> GHMDQETIDTDYDVIVLGTGITECILSGLLSVDGKKV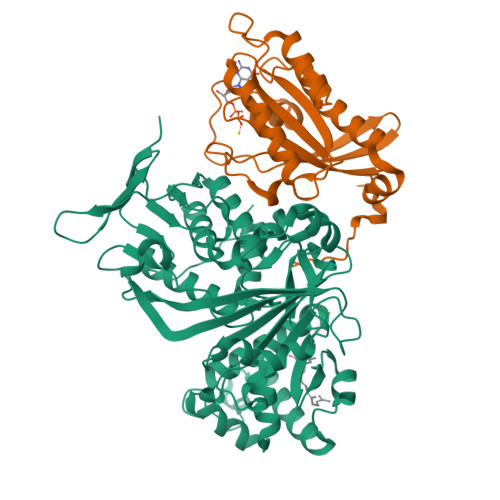LHIDKQDHYGGEAASVTLSQLYEKFKQNPISKEERESKFGKDRDWNVDLIPKFLMANGELTNILIHTDVTRYVDFKQVSGSYVFKQGKIYKVPANEIEAISSPLMGIFEKRRMKKFLEWISSYKEDDLSTHQGLDLDKNTMDEVYYKFGLGNSTKEFIGHAMALWTNDDYLQQPARPSFERILLYCQSVARYGKSPYLYPMYGLGELPQGFARLSAIYGGTYMLDTPIDEVLYKKDTGKFEGVKTKLGTFKAPLVIADPTYFPEKCKSTGQRVIRAICILNHPVPNTSNADSLQIIIPQSQLGRKSDIYVAIVSDAHNVCSKGHYLAIISTIIETDKPHIELEPAFKLLGPIEEKFMGIAELFEPREDGSKDNIYLSRSYDASSHFESMTDDVKDIYFRVTGHPLVLKQRQEQEKQ;> MNSEYDYLFKLLLIGNSGVGKSCLLLRFSDDTYTNDYISTIGVDFKIKTVELDGKTVKLQIWDTAGQERFRTITSSYYRGSHGIIIVYDVTDQESFNGVKMWLQEIDRYATSTVLKLLVGNKCDLKDKRVVEYDVAKEFADANKMPFLETSALDSTNVEDAFLTMARQIKESMSQQNLNETTQKKEDKGNVNLKGQSLTNTGGGCC> SVGEGPDTKPTARGQPAAVGRVVVLSGPSAVGKSTVVRCLRERIPNLHFSVSATTRAPRPGEVDGVDYHFIDPTRFQQLIDQGELLEWAEIHGGLHRSGTLAQPVRAAAATGVPVLIEVDLAGARAIKKTMPEAVTVFLAPPSWQDLQAR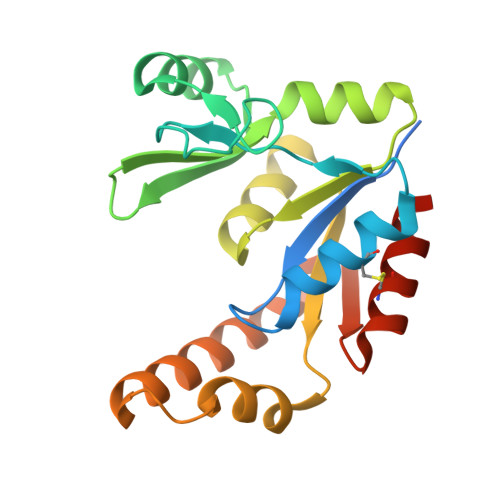LIGRGTETADVIQRRLDTARIELAAQGDFDKVVVNRRLESACAELVSLLVGTAPGSP> IVGGQECKDGECPWQALLINEENEGFCGGTILSEFYILTAAHCLYQAKRFKVRVGDRNTEQEEGGEAVHEVEVVIKHNRFTKETYDFDIAVLRLKTPITFRMNVAPACLPERDWAESTLMTQKTGIVSGFGRTHE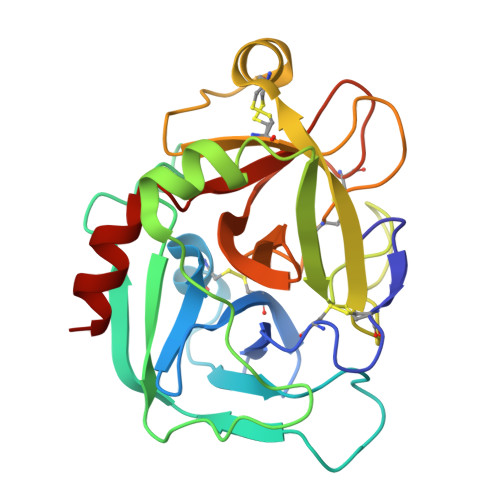KGEQSTRLKMLEVPYVDRNSCKLSSSFIITQNMFCAGYDTKQEDACQGDSGGPHVTRFKDTYFVTGIVSWGEGCARKGKYGIYTKVTAFLKWIDRSMKT>[3x]MGKVIRSLNRFGKKVGNALTSNTAKKIYSTIGKAAERFAESEIGSAAIDGLVQGSVHSIITGESYGESVKQAVLLNVLGSGEEIPDPLSPGERGIQAKLKELEDEQRNELVRLKYNDKIKEKFGKELEEVYNFMNGEANAEIEDEKQFDILNKAVTSYNKILTEEDLQMRRLATALQKEIGERTHAETVMVKEYRDKIDALKNAIEVERDGMQEEAIQEIAGMTADVLEAASEEVPLIGAGMATAVAT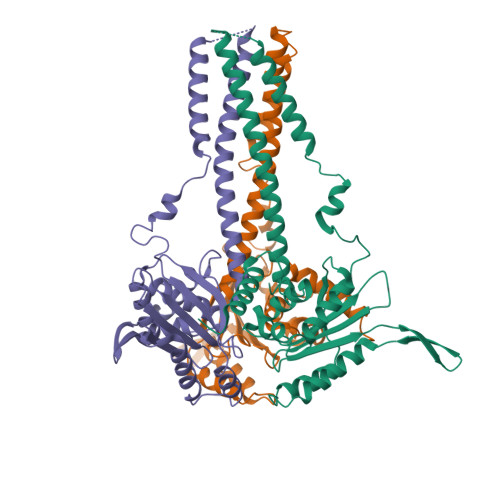GRAIEGAYKLKKVINALSGIDLTHLRTPKIEPSVVSTILEYRAKEIPDNALAVSVLSKNRAIQENHKELMHIKNEILPRFKKAMDEEKEICGIEDKVIHPKVMMKFKIPRAQQPQIHVYSAPWDSDDVFFFHCISHHHANESFFLGFDLSIDLVHYEDLTAHWHALGAAQTAAGRTLTEAYREFLNLAISNAFGTQMHTRRLVRSKTVHPIYLGSLHYDISFSDLRGNAQRIVYDDELQMHILRGPIHFQRRAILGALKFGCKVLGDRLDVPLFLRNA> EMYYST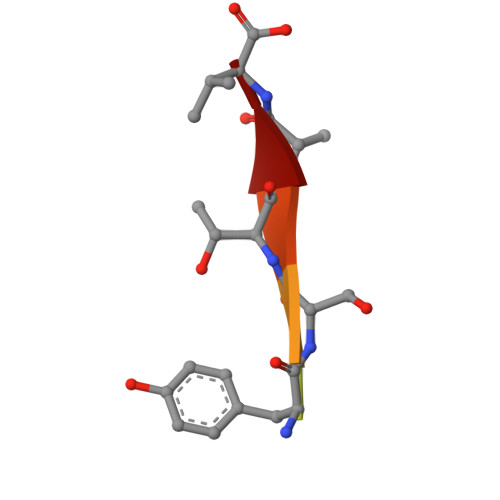AV> AMADIGSEFGHRTLASTPALWASIPCPRSELRLDLVLPSGQSFRWREQSPAHWSGVLADQVWTLTQTEEQLHCTVYRGDKSQASRPTPDELEAVRKYFQLDVTLAQLYHHWGSVDSHFQEVAQKFQGVRLLRQDPIECLFSFICSSNNNIARITGMVERLCQAFGPRLIQLDDVTYHGFPSLQALAGPEVEAHLRKLGLGYRARYVSA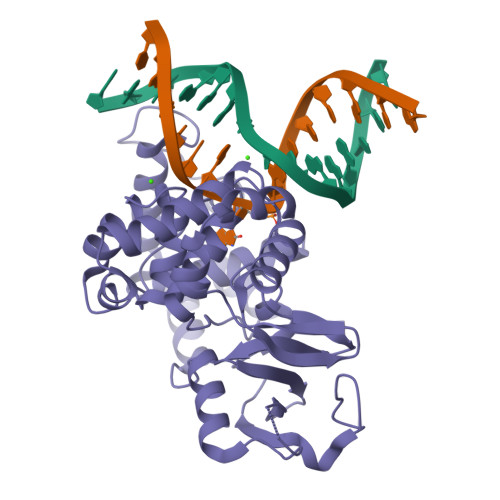SARAILEEQGGLAWLQQLRESSYEEAHKALCILPGVGTQVADCICLMALDKPQAVPVDVHMWHIAQRDYSWHPTTSQAKGPSPQTNKELGNFFRSLWGPYAGWAAAVLFSADLRQSR>[2x]MSRNCLDLYEEILTEEGTAKEATYNDLQ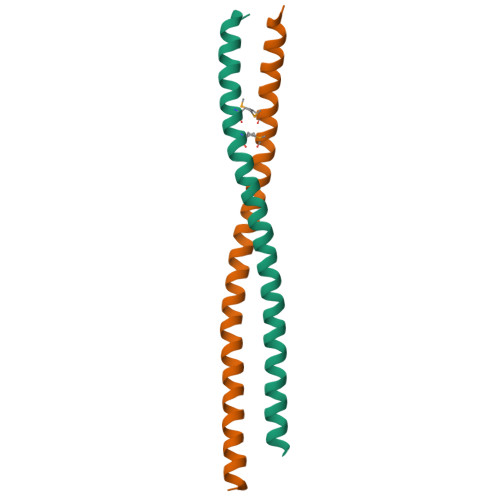VEYGKCQLQMKELMKKFKEIQAQNFSLINENQSLKKNISALIKTARVEINRKDEEISNLHLEHHHHHH>[2x]MENTENSVDSKSIKNLEPKIIHGSESMDSGISLDNSYKMDYPEMGLCIIINNKNFHKSTGMTSRSGTDVDAANLRETFRNLKYEVRNKNDLTREEIVELMRDVSKEDHSKRSSFVCVLLSHGEEGIIFGTNGPVDLKKITNFFRGDRCRSLTGKPKLFIIQAARGTEL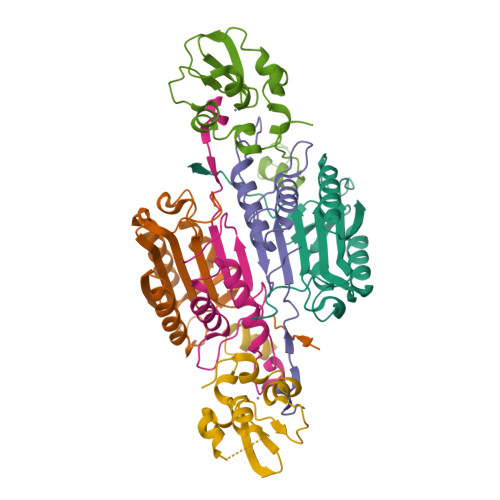DCGIETD;>[2x]SGVDDDMACHKIPVEADFLYAYSTAPGYYSWRNSKDGSWFIQSLCAMLKQYADKLEFMHILTRVNRKVATEFESFSFDATFHAKKQIPCIVSMLTKELYFYHLEHHHHHH;>GSHMRDHFALDRPSETHADYLLRTGQVVDISDTIYPRNPAMYSEEARLKSFQNWPDYAHLTPRELASAGLYYTGIGDQVQCFACGGKLKNWEPGDRAWSEHRRHFPNCFFVLGRNLNIRSE[2x]> KDDFAKLEEQFDAKLGIFALDTGTNRTVAYRPDERFAFASTIKALTVGVLLQQKSIEDLNQRITYTRDDLVNYNPITEKHVDTGMTLKELADASLRYSDNAAQNLILKQIGGPESLKKELRKIGDEVTNPERFCPELNEVNPGETQDTSTARALVTSLRAFALEDKLPSEKRELLIDWMKRNTTGDALIRAGVPDGWEVADKTGAASYGTRNDIAIIWPPKGDPVVLAVLSSRDKKDAKYDDKLIAEATK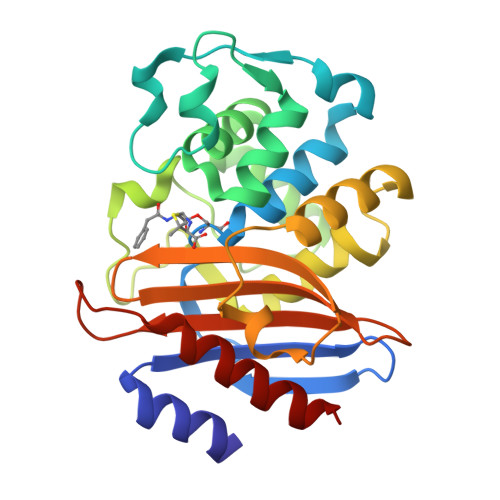VVMKALN2-AMINO-4-FLUORO-5-[(1-METHYL-1H-IMIDAZOL-2-YL)SULFANYL]-N-(1,3-THIAZOL-2-YL)BENZAMIDE | C14 H12 F N5 O S2 | 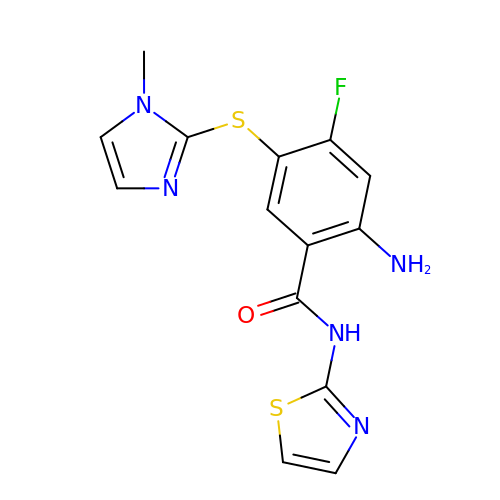YUCYMQBDBXVNCE-UHFFFAOYSA-N>MGTTTMGVKLDDATRERIKSAATRIDRTPHWLIKQAIFSYLEQLENS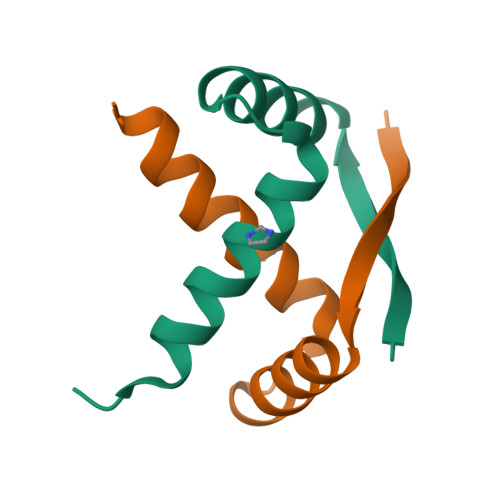DTLPE[4x]>[11x]MELLWCELNRDLPTPLYEQLYAHIKTEITEGRIGYGTKLPSKRKLADSLKLSQNTVEAAYEQLVAEGYVEVIPRKGFYVQAYEDLEYIRAPQAPGDALATKQDTIRYNFHPTHIDTTSFPFEQWRKYFKQTMCKENHRLLLNGDHQGEASFRREIAYYLHHSRGVNCTPEQVVVGAGVETLLQQLFLLLGESKVYGIED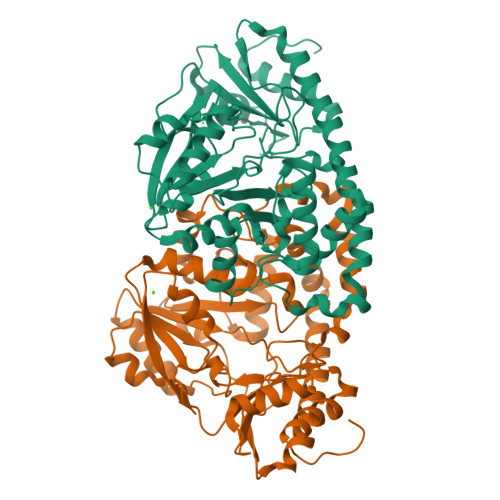PGYQLMRKLLSHYPNDYVPFQVDEEGIDVDSIVRTAVDVVYTTPSRHFPYGSVLSINRRKQLLHWAEAHENRYIIEDDYDSEFRYTGKTIPSLQSMDVHNKVIYLGAFSKSLIPSVRISYMVLPAPLAHLYKNKFSYYHSTVSRIDQQVLTAFMKQGDFEKHLNRMRKIYRRKLEKVLSLLKRYEDKLLIIGERSGLHIVLVVKNGMDEQTLVEKALAAKAKVYPLSAYSLERAIHPPQIVLGFGSIPEDELEEAIATVLNAWGFLVPRGSLEHHHHHH3-{[(9beta,14beta,16alpha,17alpha)-3,17-dihydroxyestra-1,3,5(10)-trien-16-yl]methyl}benzamide | C26 H31 N O3 | 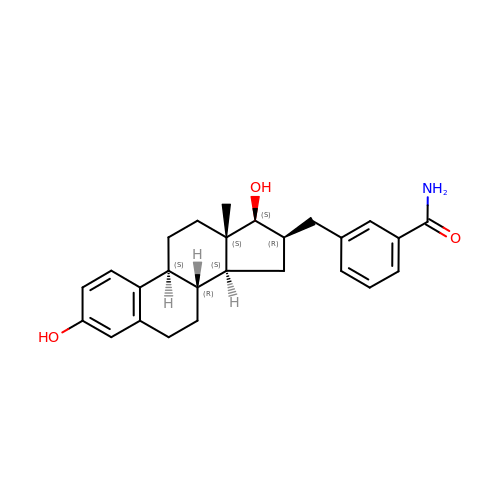RSVOVHDOLNWYER-RYZVYYIHSA-N>LEEKKVCQGTSNKLTQLGTFEDHFLSLQRMFNNCEVVLGNLEITYVQRNYDLSFLKTIQEVAGYVLIALNTVERIPLENLQIIKGNMYYENSYALAVLSNYDANKTGLKELPMRNLQEILHGAVRFSNNPALCNVESIQWRDIVSSDFLSNMSMDFQNHLGSCQKCDPSCPNGSCWGAGEENCQKLTKIICAQQCSGRCRGKSPSDCCHNQCAAGCTGPRESDCLVCRKFRDEATCKDTCPPLMLYNPTTYQMDVNPEGKYSFGATCVKKCPRNYVVTDHGSCVRACGADSYEMEEDGVRKCKKCEGPCRKVCNGIGIGEFKDSLSINATNIKHFKNCTSISGDLHILPVAFRGDSFTHTPPLDPQELDILKTVKEITGFLLIQAWPENRTDLHAFENLEIIRGRTKQHGQFSLAVVSLNITSLGLRSLKEI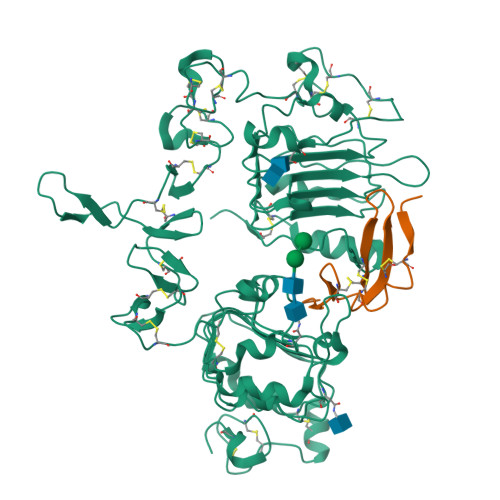SDGDVIISGNKNLCYANTINWKKLFGTSGQKTKIISNRGENSCKATGQVCHALCSPEGCWGPEPRDCVSHHHHHH[2x];>VSITKCSSDMNGYCLHGQCIYLVDMSQNYCRCEVGYTGVRCEHFFLTV[2x]> MNLTDSLQNVLSGVGTLNRYRLDIPSCPSSLDVEDFSGTEGISKIYRYDIIFTSTDRYPDAAWFLRKSATLIMGTGLLESLTEQKKVHGVITDFRRISGSEDQAQYRITLKPFISLLDKQFRTHRFFVNKSVPEVVEQILTEHGLKGWEYEFSLKRTYPKREQINQYQESDLRFIQRLLAEVGIFYFFTLHPDAQTEVIHFGDVQAALIFDKTLPVNSPSGMSDSGTDSVWALNVEHRVVESRVITNDYNHREAQNILMSVPADMTRGEGYDTSYGEVYHYRPRHTERGDKIDPAPETANFWARLDHERFLAEQTRITGKSTDASLLPAQVLTITDSTPPVLPAPLQEPVLLTQLLFTGSRKSALQVMLSAVPYSEIVCWRPPLLTRPKITGTMTARVTSAKEGDIYAWQDASGMYRVKFDADRDDKNPGQESMPVRLAKPYSGDAYGFHFPLIQGTEVAIAFEEGDPDRPYIAHALHDSRHVDHVTDKNGTRNVIRTPANNKLRMEDKRGEEHIKLSTEYGGKTQLNLGHNVDASRELRGEGAELRTDDWISI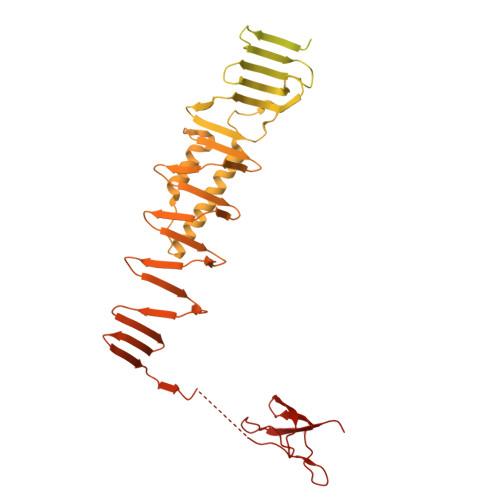RGGKGIFISADMQPQAQGKMLDMDEAIRQLEQALSLARSMAKAATAANATQGDISCQQRLNASLTDLTAPGMLLHAPDGIGMVSARALRIASGSESVGIMSGDNTDITAGQSFTVVAEGAVSLLSRNQGMQLLAAKGRVNIQAQSDDLSMSSQQNLDIQSSEGKVTVSANQELILACGGAYIKLSGGNIELGCPGQILLKSTNMQKMGPTSLDIASVEMPRGFGGGFILTDEAGVPQPSTPYRLTTAEGDILQGITDENGKTAPVNTSIPSVVKVEFGKVKIHGETE>GFQTFEGDLKWHHHNITYWIQNYSEDLPRAVIDDAFARAFALWSAVTPLTFTRVYSRDADIVIQFGVAEHGDGYPFDGKDGLLAHAFPPGPGIQGDAHFDDDELWSLGKGVGYSLFLVAAHEFGHALGLDHSSV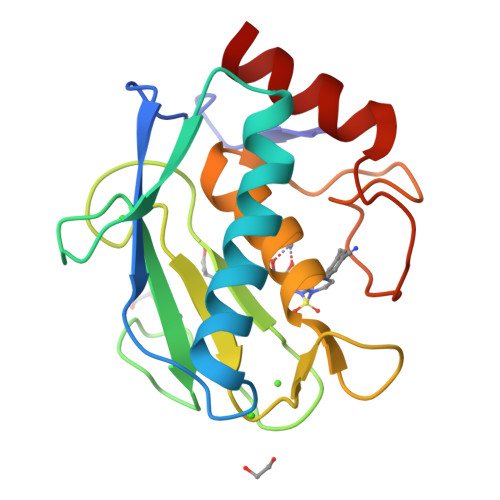PEALMYPMYRFTEGPPLHKDDVNGIRHLYG[2x]> GSHMNLKVEFFNAGTQAQSNSIYP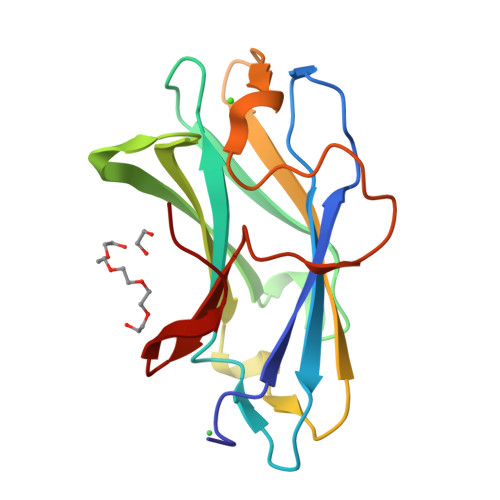KFRLTNTGSNAINLADVKLHYYFTVDGDKAQTFWCDWSPVGSSNVTGTFVKMNPTTTGADQYLEIAFSSAAGTLAANTSIEVQGRFAKSDWTNYNQADDYSFNSSATTYTSWDKVTAYSAEGLIWGIEP>[7x]MHHHHHHENL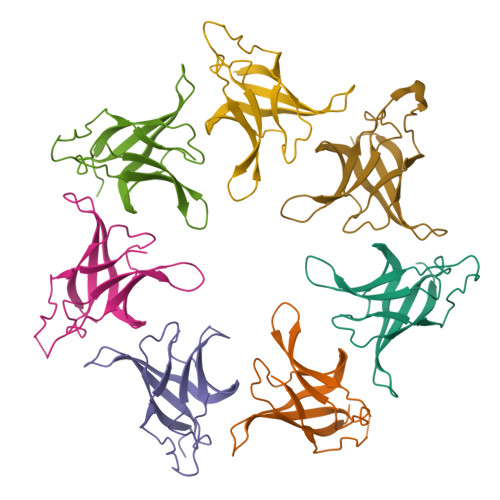YFQTSIRTEPTYTLYATFDNIGGLKARSPVSIGGVVVGRVADITLDPKTYLPRVTLEIEQRYNHIPDTSSLSIRTSGLLGEQYLALNVGFEDPELGTAILKDGDTIQDTKSA DPP III (EC 3.4.14.4; earlier names: dipeptidyl arylamidase III, dipeptidyl aminopeptidase III) is a cytosolic zinc-metallopeptidase of the M49 family. This exopeptidase catalyses the hydrolysis of the penultimate peptide bond of its oligopeptide substrates with unsubstituted N-termini, thereby sequentially removing N-terminal dipeptides. Despite a low sequence identity (17–21%), the overall structure of BtDPP III is very similar to the previously reported crystal structures of human and yeast DPP III and consists of two domains separated by a wide cleft. The catalytic zinc ion is positioned in the lower part of the upper structural domain, coordinated by His448, His453, and Glu476.

The wild-type DPP III crystals were obtained only after the initial crystallization conditions with Se-Met labelled Cys-null protein were determined. Out of more than 100 drops prepared using these four conditions, just a few crystals of the wild-type protein grew in the E2 condition of the JCSG+ screen (Molecular Dimensions, Newmarket, UK), while other drops did not yield any crystals. The structure was solved at 2.4 Å resolution using molecular replacement, with the structure of the Cys-null variant as a search model. Both proteins crystallized in space group P3121, with one molecule in the asymmetric unit. By superimposing the wild-type on the Cys-null structures, we confirmed that the replacement of cysteine residues or the incorporation of Se-Met did not change the protein structure (backbone RMSD 0.15 Å). Therefore, only the wild-type structure was considered in further discussion. The coordination of the zinc ion is square pyramidal with two water molecules in the remaining positions. In contrast, in both human and yeast DPP III, zinc exhibits a tetrahedral coordination with a single water molecule that is considered to be important for the generally accepted catalytic mechanism involving water activation by Glu461. It is interesting that in the case of BtDPP III, the corresponding Glu449 does not point toward either of the two zinc-coordinated water molecules. The superimposed protein backbones of ligand-free bacterial and ligand-free human DPP III structures gave rise to an RMSD value of 4.41 Å. Namely, human DPP III is more open than the bacterial enzyme.

> MAVTATILASCGGAKTTTAEADKFDYTVEQFADLQILRYKVPEFETLTLKQKELVYYLTQAALEGRDILFDQNGKYNLRIRRMLEAVYTNYKGDKSAPDFKNMEVYLKRVWFSNGIHHHYGMEKFVPGFSQDFLKQAVLGTDAQLLPLSEGQTAEQLCDELFPVMFDPAILAKRVNQADGEDLVLTSACNYYDGVTQQEAESFYGAMKDPKDETPVSYGLNSRLVKEDGKIQEKVWKVGGLYTQAIEKIVYWLKKAETVAENDAQKAVISKLIQFYETGSLKDFDEYAILWVKDLDSRIDFVNGFTESYGDPLGVKASWESLVNFKDLDATHRTEIISSNAQWFEDHSPVDKSFKKEKVKGVSAKVITAAILAGDLYPATAIGINLPNANWIRAHHGSKSVTIGNITDAYNKAAHGNGFNEEFVCNDEERQRIDQYGDLTGELHTDLHECLGHGSGKLLPGVDPDALKAYGSTIEEARADLFGLYYVADPKLVELKLVPDAEAYKAEYYTFLMNGLMTQLVRIEPGNNIEEAHMRNRQLIARWVFEKGAPDKVVEMVKKDGKTYVVVNDYEKVRQLFGELLAEIQRIKSTGDFEGARTLVENYAVKVDPALHAEVLARYKKLNLAPYKGFINPVYELVTDKDGNITDVTVSYNEDYVEQMLRYSKDYSPLPSVNNLEHHHHHH> GPGSTTALQEALKEKQQHIEQLLAERDLERAEVAKATSHVGEIEQELALARDGHDQHVLELEAKMDQLRTMVEAADREKVELLNQLEEE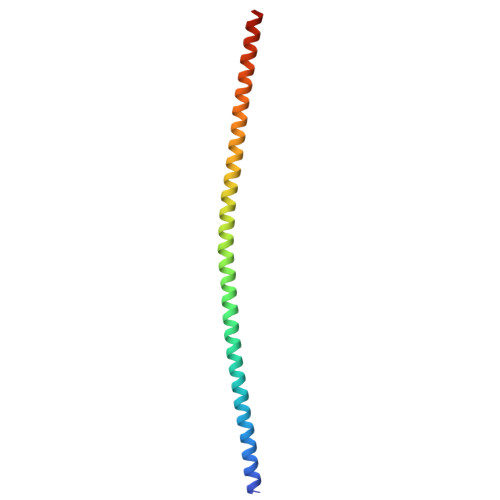KRKVEDLQFRVEEESITKGDLE> MSKPQPIAAANWKCNGSQQSLSELIDLFNSTSINHDVQCVVASTSSHLAMTKERLSHPKFVIAAQNAGNADALAS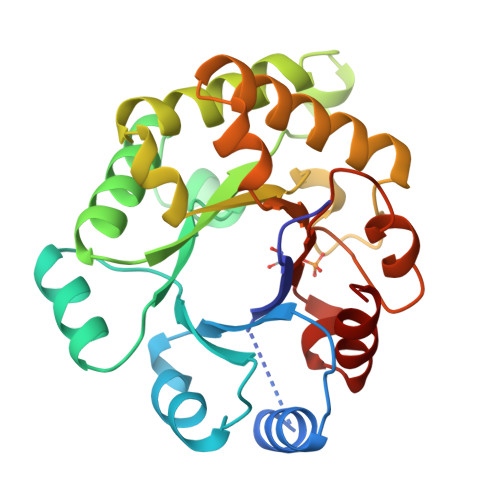LKDFGVNWIVLGHSERRAYYGETNEIVADKVAAAVASGFMVIACIGETLQERESGRTAVVVLTQIAAIAKKLKKADWAKVVIAYEPVWAIGTGKVATPQQAQEAHALIRSWVSSKIGADVAGELRILYGGSVNGKNARTLYQQRDVNGFLVGGASLKPEFVDIIKATQ> GHMSMQGPRTRPRKPIRAGEVLFAVGGWASGDAISSVERYDPQTNEWRMVASMSKRRCGVGVSVLDDLLYAVGGHDGSSYLNSVERYDPKTNQWSSDVAPTSTARTSVGVAVLGGFLYAVGGQDGVSALNIVERYDPKENKWTRVASMSTRRLGVAVAVLGGFLYAVGGSDGT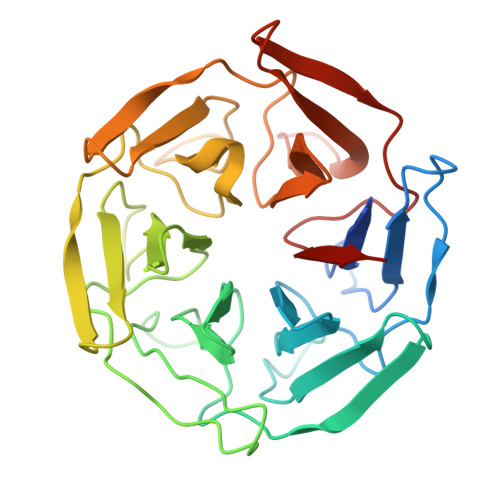SPLNTVERYNPQENRWHTIAPMGTRRKHLGCAVYQDMIYAVGGRDDTTELSSAERYNPRTNQWSPVVAMTSRRSGVGLAVVNGQLMAVGGFDGTTYLKTIEVFDPDANTWRLYGGMNYRRLGGGVGVIKMTHAE> GAMGMKVDVGPDPSLVYRPDVDPEMAKSKDSFRNYTSGPLLDRVFTTYKLMHTHQTVDFVSRKRIQYGSFSYKKMTIMEAVGMLDDLVDESDPDVDFPNSFHAFQTAEGIRKAHPDKDWFHLVGLLHDLGKIMALWGEPQWAVVGDTFPVGCRPQASVVFCDSTFQDNPDLQDPRYSTELGMYQPHCGLENVLMSWGHDEYLYQMMKFNKFSLPSEAFYMIRFHSFYPWHTGGDYRQLCSQQDLDMLPWVQEFNKFDLYTKCPDLPDVESLRPYYQGLIDKYCPGTLS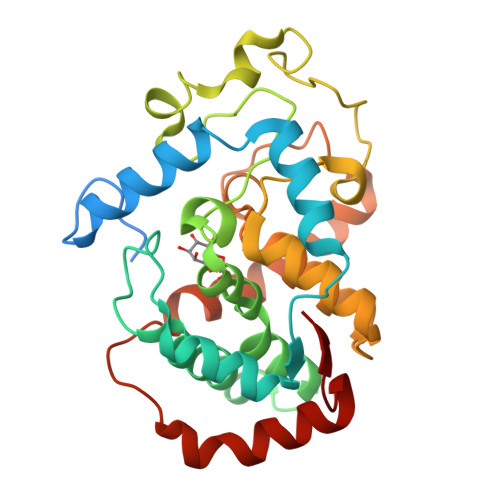W> MIASINDTDMDTDDNMSQARRNRRNRPPARPSAQTQMAAVDMLQTINTAASQTAASLLINDITPNKTESLKILSTQSVGARSLLEPMQANASTIKLNRIETVNVLDFL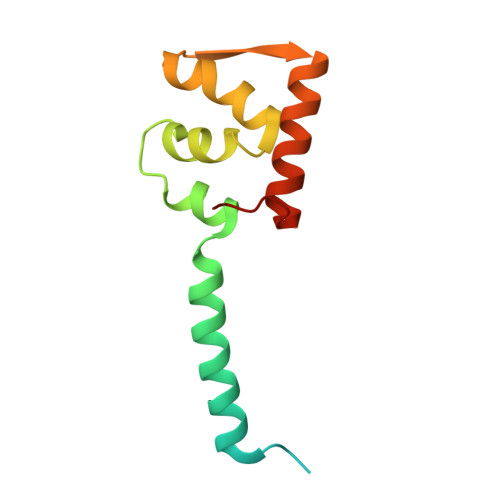GSVYDNTIQVIVTE>[3x]MATRIAILGAGPS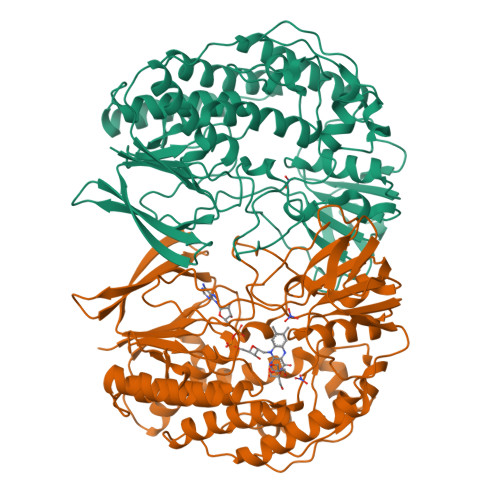GMAQLRAFQSAQEKGAEIPELVCFEKQADWGGQWNYTWRTGLDENGEPVHSSMYRYLWSNGPKECLEFADYTFDEHFGKPIASYPPREVLWDYIKGRVEKAGVRKYIRFNTAVRHVEFNEDSQTFTVTVQDHTTDTIYSEEFDYVVCCTGHFSTPYVPEFEGFEKFGGRILHAHDFRDALEFKDKTVLLVGSSYSAEDIGSQCYKYGAKKLISCYRTAPMGYKWPENWDERPNLVRVDTENAYFADGSSEKVDAIILCTGYIHHFPFLNDDLRLVTNNRLWPLNLYKGVVWEDNPKFFYIGMQDQWYSFNMFDAQAWYARDVIMGRLPLPSKEEMKADSMAWREKELTLVTAEEMYTYQGDYIQNLIDMTDYPSFDIPATNKTFLEWKHHKKENIMTFRDHSYRSLMTGTMAPKHHTPWIDALDDSLEAYLSDKSEIPVAKEALEHHHHHH> MKERRASQKLSSKSIMDPNQNVKCKIVVVGDSQCGKTAL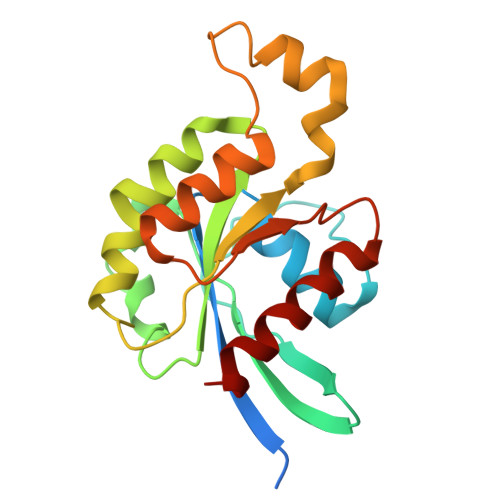LHVFAKDCFPENYVPTVFENYTASFEIDTQRIELSLWDTSGSPYYDNVRPLSYPDSDAVLICFDISRPETLDSVLKKWKGEIQEFCPNTKMLLVGCKSDLRTDVSTLVELSNHRQTPVSYDQGANMAKQIGAATYIECSALQSENSVRDIFHVATLACVNK> CUGCU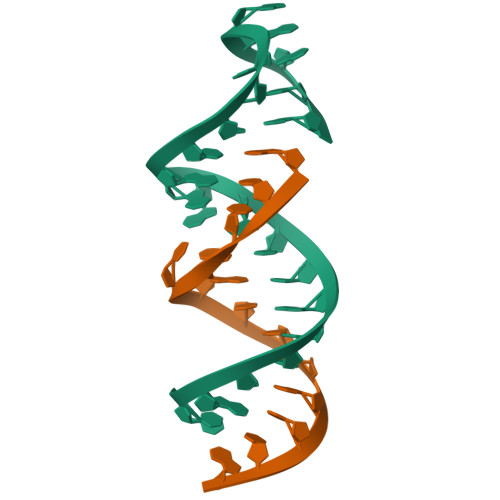GGCUAAGGCCCGAAAGG;> GCUAUGCCUGCUG>MAKVLCVLYDDPVDGYPKTYARDDLPKIDHYPGGQTLPTPKAIDFTPGQLLGSVSGELGLRKYLESNGHTLVVTSDKDGPDSVFERELVDADVVISQPFWPAYLTPERIAKAKNLKLALTAGIGSDHVDLQSAIDRNVTVAEVTYCNSISVAEHVVMMILSLVRNYLPSHEWARKGGWNIADCVSHAYDLEAMHVGTVAAGRIGLAVLRRLAPFDVHLHYTDRHRLPESVEKELNLTWHATREDMYPVCDVVTLNCPLHPETEHMINDETLKLFKRGAYIVNTARGKLCDRDAVARALESGRLAGYAGDVWFPQPAPKDHPWRTMPYNGMTPHISGTTLTAQARYAAGTREILECFFEGRPIRDEYLIVQGGALAG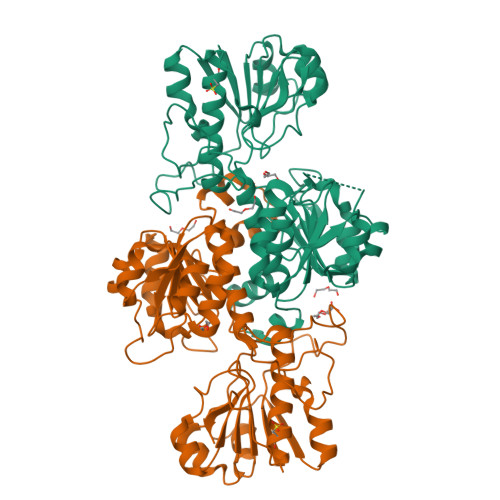TGAHSYSKGNATGGSEEAAKFKKAV[4x]2-hydroxyethyl 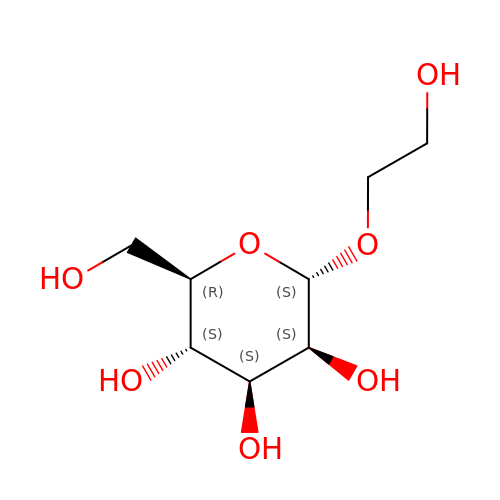alpha-D-mannopyranoside | C8 H16 O7 | SMORULFPMBCEPX-HEIBUPTGSA-N>[4x]SNAMIRDYLEDKPLIDESVFVAKSADVIGNVKIGKDSS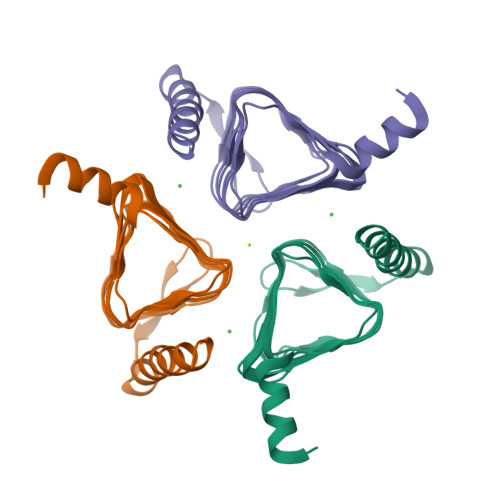IWYNAVVRGDEGPITIGENTNIQDCSIVHGDTETIIGNNVTVGHRSIVHGCKISDNVLIGMGSIILDNAEIGEYTLIGAGTLITSNKKFPPGVLIMGSPGKVVRELTEEDKKYIDESYEWYLEAAQNQKY>[6x]QETLVRPKPLLLKLLKSVGAQKDTYTMK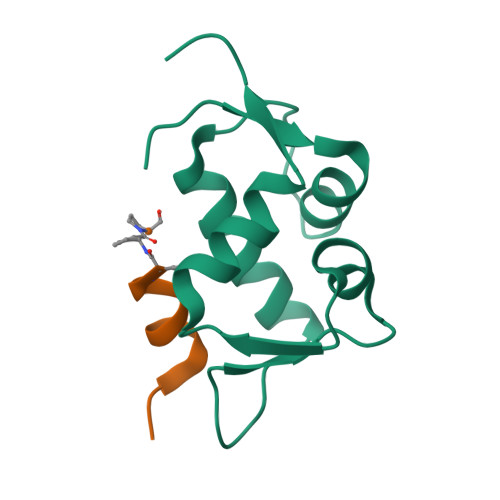EVLFYLGQYIMTKRLYDEKQQHIVYCSNDLLGDLFGVPSFSVKEHRKIYTMIYRNLVVVNQQ;>ATSFAEYWALLXPA[6x]> GAASNKSTSSAMSGSHQDLSVIQPIVKDCKEADLSLYNEFRLWKDEPTMDRTCPFLDKIYQEDIFPCLTFSKSELASAVLEAVENNTLSIE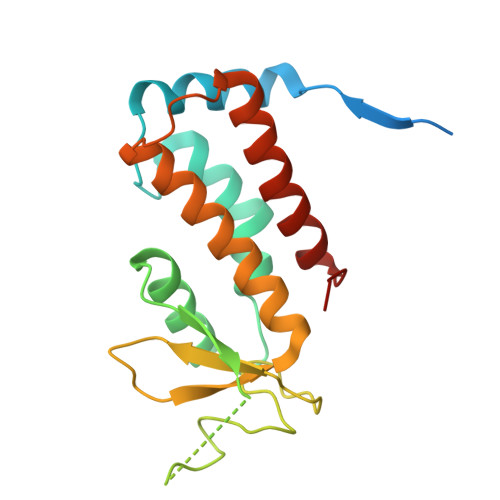PVGLQPIRFVKASAVECGGPKKCALTGQSKSCKHRIKLGDSSNYYYISPFCRYRITSVCNFFTYIRYIQQGLVKQQDVDQMFWEVMQLRKEMSLAKLGYFKEEL>MRGSHHHHHHSGQRMGMVIGIKPEHIDEYKRLHAAVWPAVLARLAEAHVRNYSIFLREPENLLFGYWEYHGTDYAADMEAIAQDPETRRWWTFCGPCQEPLASRQPGEHWAHME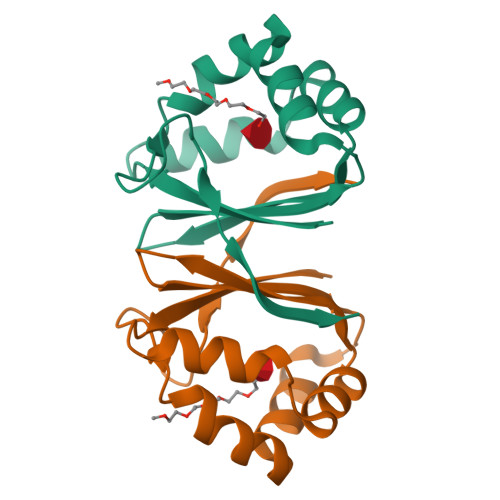EVFHVD[2x]>MGTGKELVLALYDYQEKSPREVTMKKGDILTLLNSTNKDWWKVEVNDRQGFVPAAYVKKLDPAQSASRENLGG[2x];>PPPV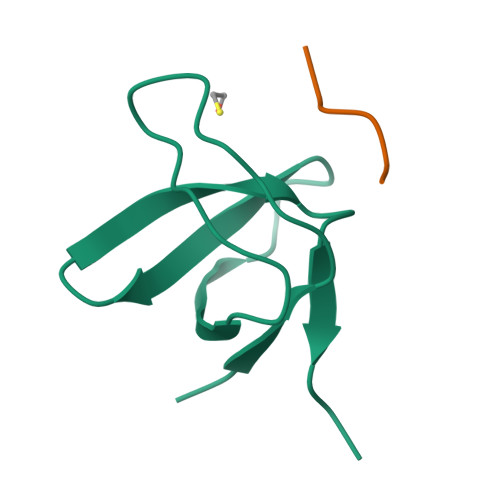PPYSAG[2x]> 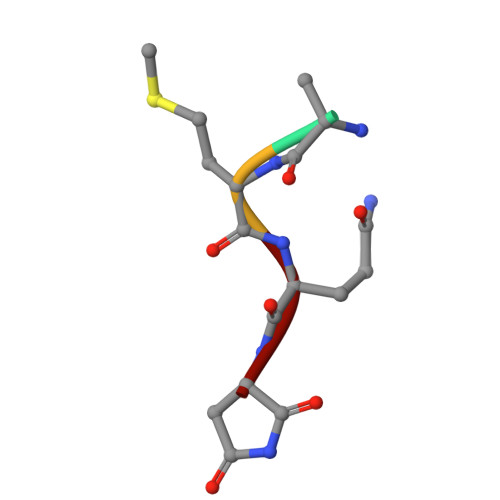QMQN>[2x]SNAPVVSAAPLATRGLKTI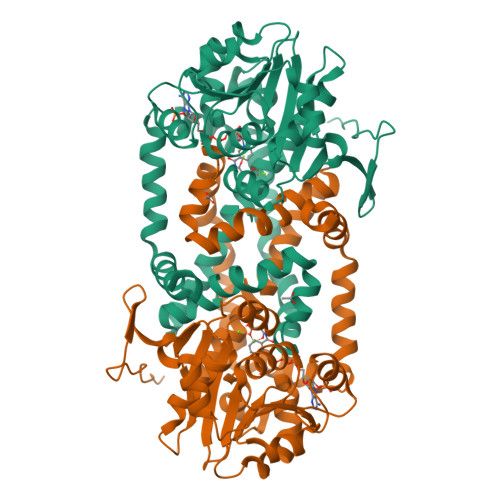NFGGTEEVVHERADWPREKLLEYFKNDTMALIGYGSQGYGQGLNLRDNGLNVIIGVRKNGASWKAAIEDGWVPGENLFDVKEAITKGTIIMNLLSDAAQSETWPDLKPLITEGKTLYFSHGFSPVFKDLTKVEPPSNVDVILAAPKGSGRTVRSLFLEGRGINSSYAVWNDVTGKAEEKAIAMAVAIGSGYVYQTTFEREVNSDLYGERGCLMGGIHGMFLAQYEVLRENGHTPSEAFNETVEEATQSLYPLIGKYGMDYMYDACSTTARRGALDWYPRFKDALKPVFVELYESVKNGTETQRSLDFNGAPDYRERLEEELETIRNMEIWKVGKEVRKLRPENQ> MGYTVGLDIGVASVGVAVLDENDNIVEAVSNIFDEADTSNNKVRRTLREGRRTKRRQKTRIEDFKQLWETSGYIIPHKLHLNIIELRNKGLTELLSLDELYCVLLSMLKHRGISYLEDADDGEKGNAYKKGLAFNEKQLKEKMPCEIQLERMKKYGKYHGEFIIEINDEKEYQSNVFTTKAYKKELEKIFETQRCNGNKINTKFIKKYMEIYERKREYYIGPGNEKSRTDYGIYTTRTDEEGNFIDEKNIFGKLIGKCSVYPEEYRASSASYTAQEFNLLNDLNNLKINNEKLTEFQKKEIVEIIKDASSVNMRKIIKKVIDEDIEQYSGARIDKKGKEIYHTFEIYRKLKKELKTINVDIDSFTREELDKTMDILTLNTERESIVKAFDEQKFVYEENLIKKLIEFRKNNQRLFSGWHSFSYKAMLQLIPVMYKEPKEQMQLLTEMNVFKSKKEKYVNYKYIPENEVVKEIYNPVVVKSIRTTVKILNALIKKYGYPESVVIEMPRDKNSDDEKEKIDMNQKKNQEEYEKILNKIYDEKGIEITNKDYKKQKKLVLKLKLWNEQEGLCLYSGKKIAIEDLLNHPEFFEIDHIIPKSISLDDSRSNKVLVYKTENSIKENDTPYHYLTRINGKWGFDEYKANVLELRRRGKIDDKKVNNLLCMEDITKIDVVKGFINRNLNDTRYASRVVLNEMQSFFESRKYCNTKVKVIRGSLTYQMRQDLHLKKNREESYSHHAVDAMLIAFSQKGYEAYRKIQKDCYDFETGEILDKEKWNKYIDDDEFDDILYKERMNEIRKKIIEAEEKVKYNYKIDKKCNRGLCNQTIYGTREKDGKIHKISSYNIYDDKECNSLKKMINSGKGSDLLMYNNDPKTYRDMLKILETYSSEKNPFVAYNKETGDYFRKYSKNHNGPKVEKVKYYSGQINSCIDISHKYGHAKNSKKVVLVSLNPYRTDVYYDNDTGKYYLVGVKYNHIKCVGNKYVIDSETYNELLRKEGVLNSDENLEDLNSKNITYKF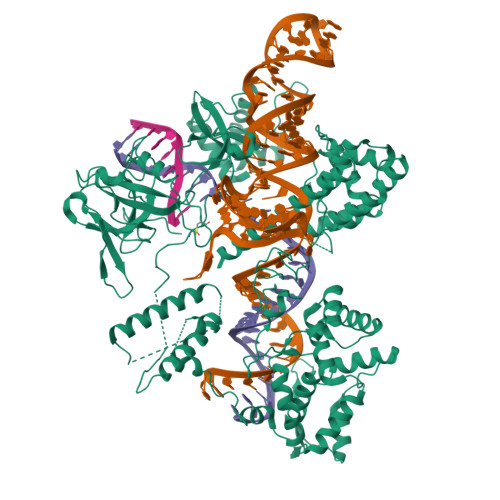SLYKNDIIQYEKGGEYYTERFLSRIKEQKNLIETKPINKPNFQRKNKKGEWENTRNQIALAKTKYVGKLVTDVLGNCYIVNMEKFSLVVDK Galectins are β-galactoside-binding lectins known primarily from animals and fungi. The fungus C. cinerea expresses several fruiting body lectins including two isogalectins, CGL1 and CGL2, and a galectin-related lectin, CGL3. In agreement with this hypothesis, we demonstrate that the C. cinerea galectin CGL2 exhibited a pronounced toxicity towards the model nematode C. elegans. Based on a number of approaches, including the use of E. coli expressing these fungal lectins to mimic the in vivo situation, we conclude that this nematotoxicity is dependent on the specific interaction between these proteins and a β-galactoside on the core of N-glycans in the C. elegans intestine.

Based on these results, the specificity of CGL2 for β-galactosides and the reported capping of core α1,6-fucose on C. elegans N-glycans with galactose residues in β1,4-configuration, we hypothesized that binding of CGL2 to this Galβ1,4Fucα1,6 epitope was required for its nematotoxicity. In order to provide biochemical and structural evidence for the interaction between CGL2 and this nematode-specific β-galactoside, the trisaccharide Galβ1,4Fucα1,6GlcNAc was chemically synthesized with a linker at the reducing end and used as ligand in in vitro binding experiments with affinity-purified CGL2. Isothermal titration microcalorimetry measurements confirmed binding of this trisaccharide to CGL2 and suggested a dissociation constant of approximately 100 µM. The molecular basis of this interaction was investigated by determining the X-ray structure of cocrystals between CGL2 and the trisaccharide at 1.5 Å resolution. A major difference between these structures lies in the orientation of the preceding monosaccharide subunits to the protein, e.g. the plane of Glc in lactose is perpendicular to the plane of Fuc in the trisaccharide. Due to the low number of direct contacts, there seems to exist a high degree of flexibility on the side of CGL2 with regard to the identity of this monosaccharide subunit. The only constraint is the orientation of the 3′ (in glucose and fucose) or 4′ (in GalNAc) OH of the linked monosaccharide to allow interaction with the conserved carbohydrate-coordinating residues, Arg55 and Glu75. In addition, these hydroxyl groups make additional contact to Arg77 in case of Glc (in lactose) and Fuc (in Galβ1,4Fucα1,6GlcNAc) but not in case of GalNAc (in Thomsen-Friedenreich antigen). In an in vivo context, the CGL2 epitope is part of a larger N-glycan structure, which may indeed have a higher affinity towards the lectin than the trisaccharide tested here.

>[4x]MLYHLFVNNQVKLQNDFKPESVAAIRSSAFNSKGGTTVFNFLSAGENILLHISIRPGENVIVFNSRLKNGAWGPEERIPYAEKFRPPNPSITVIDHGDRFQIRFDYGTSIYYNKRIKENAAAIAYNAENSLFSSPVTVDVHGLLPPLPPA>[4x]MTPKKNISKGAVLHEKPMTVMVLTATEPFNYKEGKENMFHATVATESQYYRVKVFNMDLKEKFTENKFITISKYFNSSGILEINETATVSEAAPNQMFEVPK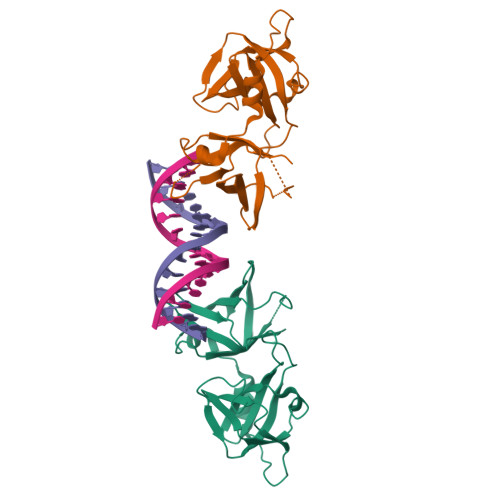NIIRSAKETLKISKIKELDSGTLIYGVFAVEKKKVNDKSITFKIKDNEDNIKVVWDKEQHNINYEKGDKLQLFSFHLRKGNGKPILHSGNHSFIKG>GSHMMPQLQFKDAFWCRDFTAHTGYEVLLQRLLDGRKMCKDMEELLRQRAQAEERYGKELVQIARKAGGQTEINSLRASFDSLKQQMENVGSSHIQLALTLREELRSLEEFRERQKEQRKKYEAVMDRVQKSKLSLYKKAMESKKTYEQKCRDADDAEQAFERISANGHQKQVEKSQNKARQCKDSATEAERVYRQSIAQLEKVRAEWEQEHRTTCEAFQLQEFDRLTILRNA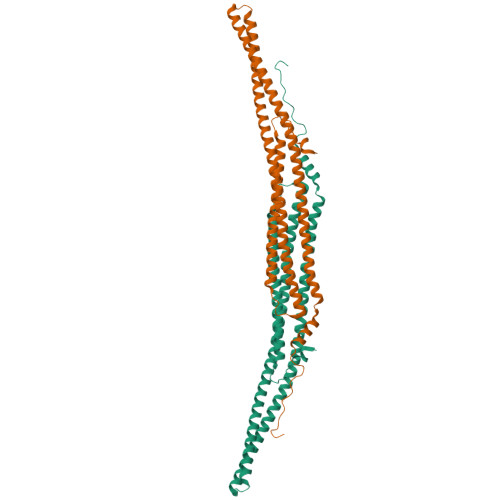LWVHSNQLSMQCVKDDELYEEVRLTLEACSIDADIDSFIQAKSTGTEPPAPVPYQNYYD[2x]>[6x]MSLDQETVGNVVLLAIVTLISVVQNGFFAHKVEHESRTQNGRSFQRTGTLAFERVYTANQNCVDAYPTFLAVLWSAGL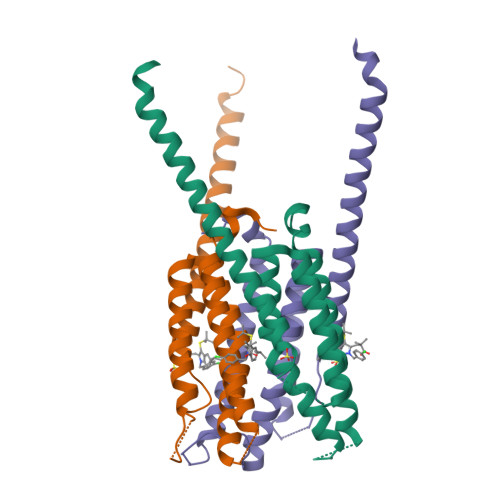LCSQVPAAFAGLMYLFVRQKYFVGYLGERTQSTPGYIFGKRIILFLFLMSVAGIFNYYLIFFFGSDFENYIATISTTISPLLLIPEGHHHHHH> AIGQKLPPFSYAYTELEAIMYALGVGASIKDPKDLKFIYEGSSDFSCLPTFGVIIGQKSMMVLHGEQYLELYKPLPRAGKLKCEAVVADVLVVIIMDVYSYSEKELICHNQFSLFLSDKVKVAVAIPNRPPDAVLTDTTSLNQAALYRLSGDWNPLHIDPNFASLAGFDKPILHGLCTFGFSARRVLQQFADNDVSRFKAV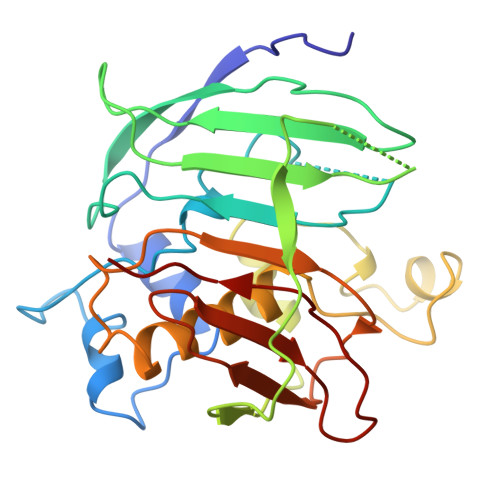KARFAKPVYPGQTLQTEMWKEGNRIHFQTKVQETGDIVISNAYVDLA> ECLPGSSPCTDALTCIKADLFCDGEVNCPDGSDEDNKMCATVCDGRFLLTGSSGSFQATHYPKPSETSVVCQWIIRVNQGLSIKLSFDDFNTYYTDILDIYEGVGSSKILRASIWETNPGTIRIFSNQVTATFLIESDESDYVGFNATYTAFNSSELNNYEKINCNFEDGFCFWVQDLNDDNEWERIQGSTFSPFTGPNFDHTFGNASGFYISTPTGPGGRQERVGLLSLPLDPTLEPACLSFWYHMYGENVHKLSINISNDQNMEKTVFQKEGNYGDNWNYGQVTLNETVKFKVAFNAFKNKILSDIALDDISLTYGICNGSLYPEPTLVPTPPPELPTDCGGPFELWEPNTTFSSTNFPNSYPNLAFCVWILNAQKGKNIQLHFQEFDLENINDVVEIRDGEEADSLLLAVYTGPGPVKDVFSTTNRMTVLLITND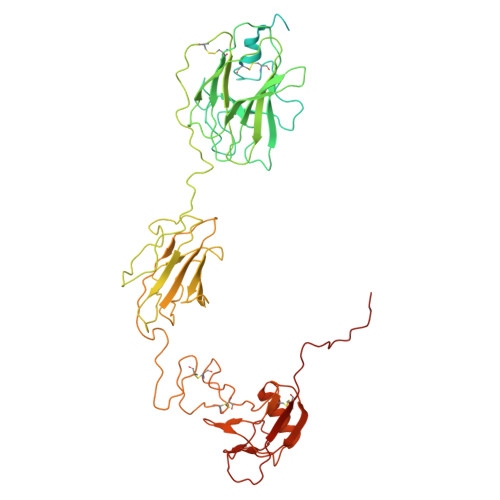VLARGGFKANFTTGYHLGIPEPCKADHFQCKNGECVPLVNLCDGHLHCEDGSDEADCVRFFNGTTNNNGLVRFRIQSIWHTACAENWTTQISNDVCQLLGLGSGNSSKPIFPTDGGPFVKLNTAPDGHLILTPSQQCLQDSLIRLQCNHKSCGKKLAAQDITPK> MSQSNRELVVDFLSYKLSQKGYSWSQFMAAVKQALREAGDEFELRYRRAFSDLTSQLHITPGTAYQSFEQVVNELFRDGVNWGRIVAFFSFGGALCV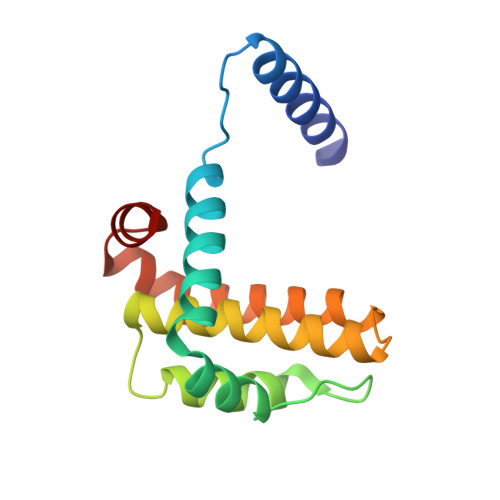ESVDKEMQVLVSRIAAWMATYLNDHLEPWIQENGGWDTFVELYG>[4x]GPLGSPGIPMSLLATVGPTGGVKNRLDIVDFVRDEKFFTLYVRALQAIQDKDQADYSSFFQLSGIHGLPFTPWAKPKDTPTVPYESGYCTHSQVLFPTWHRVYVSIYEQVLQEAAKGIAKKFTVHKKEWAQAAEDLRQPYWDTGFALVPPDEIIKLEQVKITNYDGTKITVRNPILRYSFHPIDPSFNGYPNFDTWRTTVRNPDADKKENIPALIAKLDLEADSTR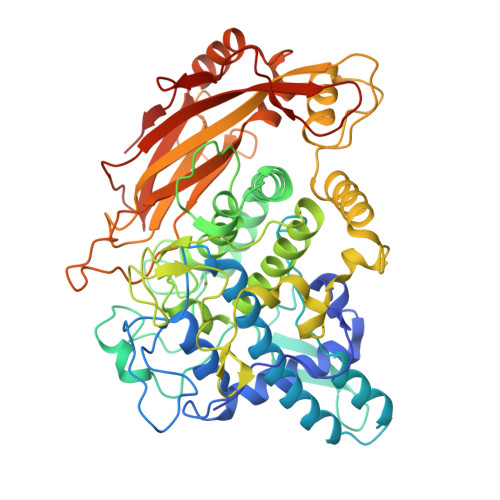EKTYNMLKFNANWEAFSNHGEFDDTHANSLEAVHDDIHGFVGRGAIRGHMTHALFAAFDPIFWLHHSNVDRHLSLWQALYPGVWVTQGPEREGSMGFAPGTELNKDSALEPFYETEDKPWTSVPLTDTALLNYSYPDFDKVKGGTPDLVRDYINDHIDRRYGIKKSEGGKNPALDLLSDFKGVTHDHNEDLKMFDWTIQASWKKFELDDSFAIIFYFAADGSTNVTKENYIGSINIFRGTTPTNCANCRTQDNLVQEGFVHLDRFIARDLDTFDPQAVHRYLKEKKLSYKVVADDHSVTLKSLRIRVQGRPLHLPPGVSFPRLDKNIPIVNFDDVLDLVTGVVNIGLT>GSHV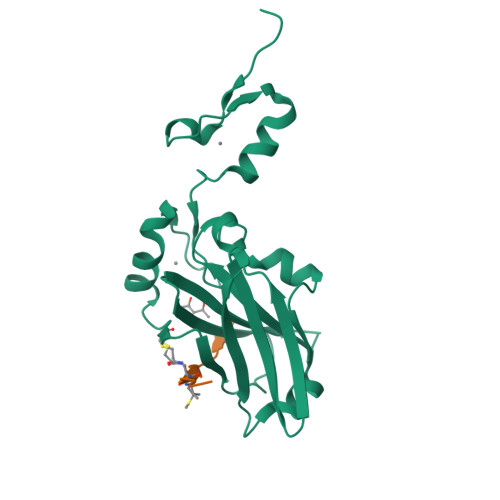ANSVLFPCKYASSGCEITLPHTEKADHEELCEFRPYSCPCPGASCKWQGSLDAVMPHLMHQHKSICTLQGEDIVFLATDINLPGAVDWVMMQSCFGFHFMLVLEKQEKYDGHQQFFAIVQLIGTRKQAENFAYRLELNGHRRRLTWEATPRSIHEGIATAIMNSDCLVFDTSIAQLFAENGNLGINVTISMC[2x];>XKLRPVXMVRPWVR[2x]> SEAS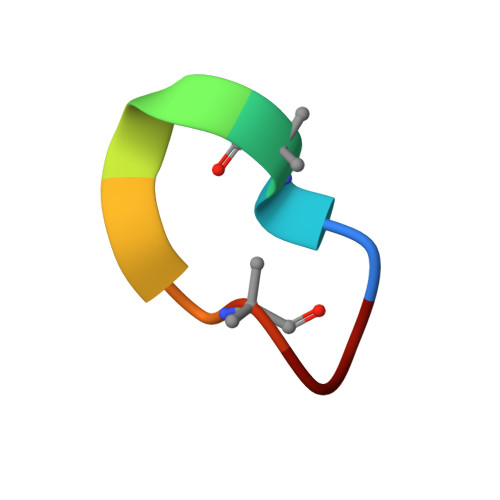LSEASL> WRDSSGY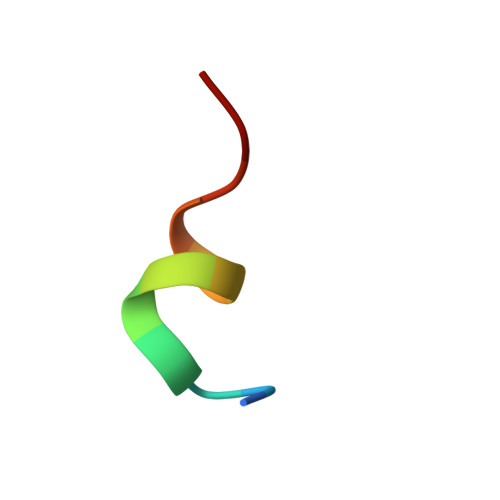VMGPW> MAKRKIQRYVRKDGKCNVHHGNVRETYRYLTDIFTTLVDLKWRFNLLIFVMVYTVTWLFFGMIWWLIAYIRGDMDHIEDPSWTPCVTNLNGFVSAFLFSIETETTIGYGYRVITDKCPEGIILLLIQSVLGSIVNAFMVGCMFVKISQPKKAAETLVFSTHAVISMRDGKLCLMFRVGDLRNSHIVEASIRAKLIKSKQTSEGEFIPLNQTDINVGYYTGDDRLFLVSPLIISHEINQQSPFWEISKAQLPKEELEIVVILEGMVEATGMTCQARSSYITSEILWGYRFTPVL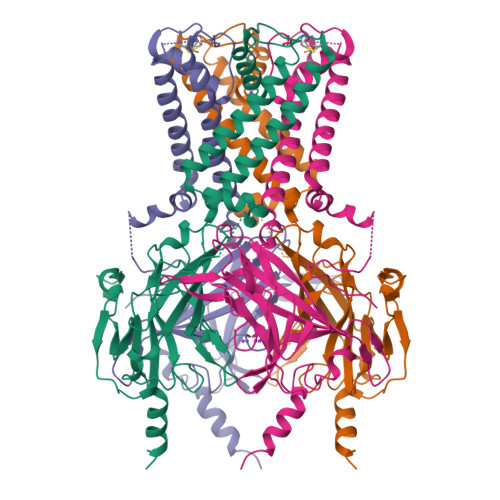TLEDGFYEVDYNSFHETYETSTPSLSAKELAELANRAESNSLEVLFQ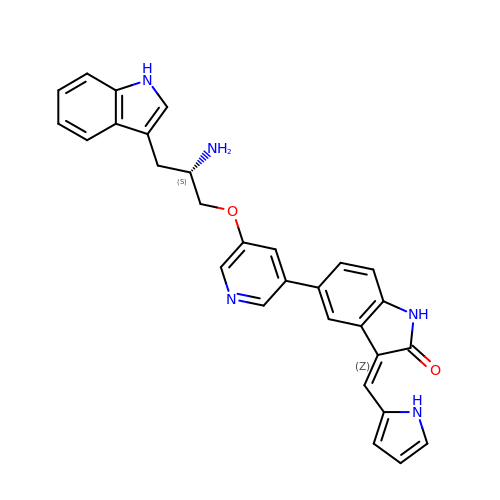5-{5-[(S)-2-AMINO-3-(1H-INDOL-3-YL)-PROPOXYL]-PYRIDIN-3-YL}-3-[1-(1H-PYRROL-2-YL)-METH-(Z)-YLIDENE]-1,3-DIHYDRO-INDOL-2-ONE | C29 H25 N5 O2 | DQMKXCKXZQEVJU-VHLXNKDGSA-N> GPKKTDPELAEKINEMLDVILE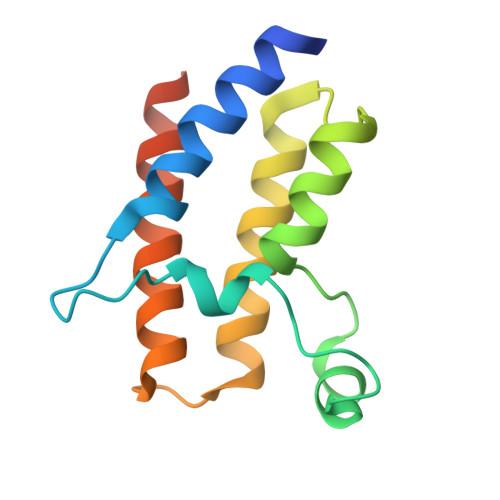YKNEDGELIADVFQTLPTRKELPDYYQVISKPMDFDRINKKIETGRYTVMEELNDDMNLLVNNAQTYNEEGSEIYVSSETIGKLWKEQYDKFMNPPKPVEE> GAMKTVGYAIVGTGYFGAELGRIMKEQEGARIVAVLDPENGQTIAEELDCDVETDLDTLYSREDVEAVIVATPNYLHKEPVIKAAEHGVNVFCEKPIALSYQDCDEMVRTCQEHGVIFMAGHVMNFFHGVRYAKKLINDGVIGKVLYCHSARNGWEEQQPTISWKKIREKSGGHLYHHIHELDCVQFLMGGMPEEVTMTGGNVAHQGEAFGDEDDMLFVNMQFSDNRYAVLEWGSA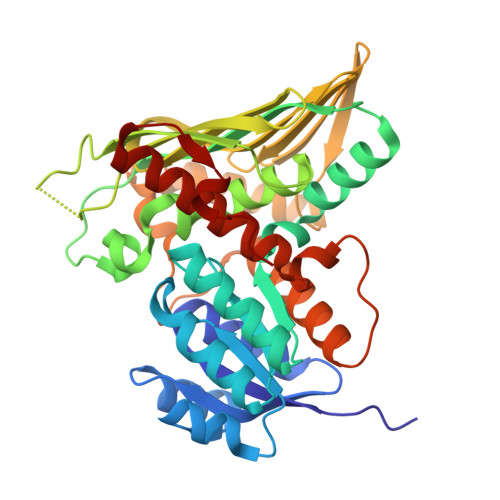FHWPEHYVLIQGTKGAIKIDMCDCGGTLKVDGREEHFLVHESQEEDDDRTRIYHGTEMDGAIMYGKPGKKPPMWLHSIMKNEMKYLNGILHGKEVDDEFRPLLTGEAARAAIATADACTKSRFEDRKVKLSEIIGEGS> GPGSEFLTEENFRRLQAEHDRQAKELFLLRKTLEEMELRIETQKQTLNARDESIKKLLEMLQSKGL;> GPGSKSSISSISGRDDLMDYHRRQREERLREQEMERLERQRLETILSLCAEYTKPDSRLSTGTTVEDVQKINK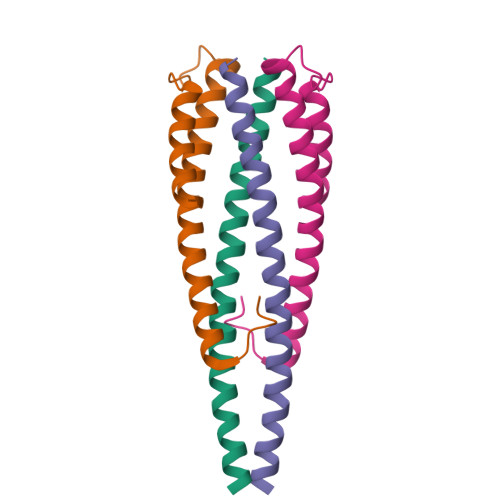ELEKLQLSD> LGTNYLLSGQTLDTEGHLKNGDFDLVMQDDCNLVLYNGNWQSNTANNGRDCKLTLTDYGELVIKNGDGSTVWK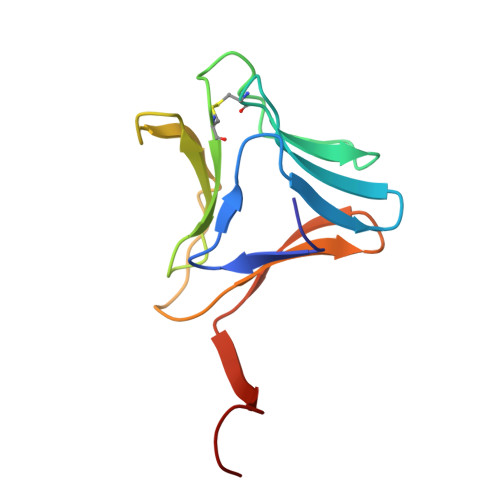SGAQSVKGNYAAVVHPDGRLVVFGPSVFKIDPWVRG>GSHMTHFSQQDNFSVAARVLGALFYYAPESAEAAPLVAVLTSDGWETQWPLPEASLAPLVTAFQTQCEETHAQAWQRLFVGPWALPSPPWGSVWLDRESVLFGDSTLALRQWMREKGIQFEMKQNEP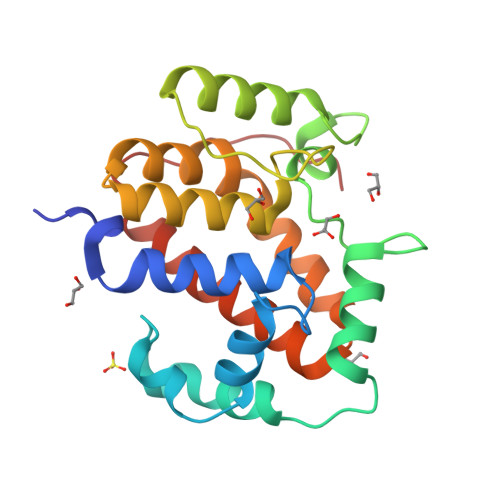EDHFGSLLLMAAWLAENGRQTECEELLAWHLFPWSTRFLDVFIEKAEHPFYRALGELARLTLAQWQSQLLIPVAVKPLFR[8x]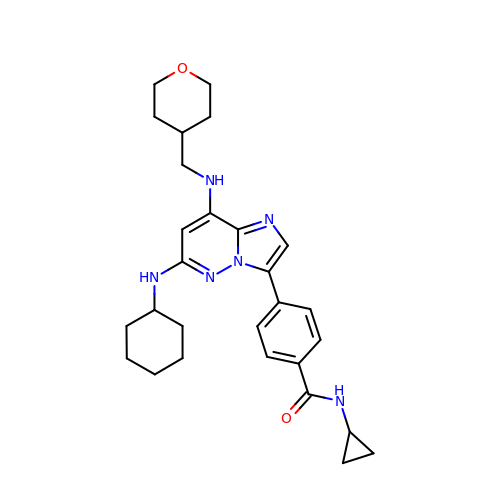4-{6-(cyclohexylamino)-8-[(tetrahydro-2H-pyran-4-ylmethyl)amino]imidazo[1,2-b]pyridazin-3-yl}-N-cyclopropylbenzamide | C28 H36 N6 O2 | ZOSFYOBMRYUXAN-UHFFFAOYSA-N> MTIGSMENVEVFTSEGKGRGLKATKEFWAADVIFAERAYSAVVFDSLINFVCHTCFKRQEKLHRCGQCKFAHYCDRTCQKDAWLNHKNECAAIKKYGKVPNENIRLAARIMWRVEREGTGLTEGCLVSVDDLQNHVEHFGEEEQKELRVDVDTFLQYWPPQSQQFSMQYISHIFGVINCNGFTLSDQRGLQAVGVGIFPNLGLVNHDCWPNCTVIFNNGNHEAVKSMFHTQMRIEL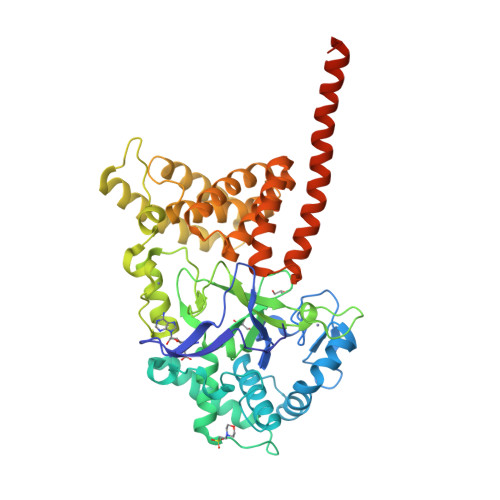RALGKISEGEELTVSYIDFLHLSEERRRQLKKQYYFDCSCEHCQKGLKDDLFLAAKEDPKPSQEVVKEMIQFSKDTLEKIDKARSEGLYHEVVKLCRECLEKQEPVFADTNLYVLRLLSIASEVLSYLQAYEEASHYARRMVDGYMKLYHHNNAQLGMAVMRAGLTNWHAGHIEVGHGMICKAYAILLVTHGPSHPITKDLEAMRMQTEMELRMFRQNEFMYHKMREAALNNQPMQVMAEPSNEPAPALFHKKQ>MSISSLLEKNIYNVHNKSNTLTNVPANPTGNTNTVWSNSNFTPPHLMYGASDITQAIGNISLTTGSFSLSLSGPWASPLVQNVAYTKINNLVNLTFPPFQANATSSAVINSAIGA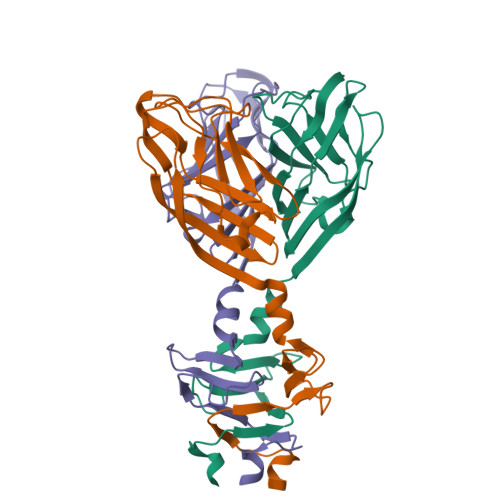LPADLRPTTNIQVDFEIFVIDDGNRPVNPGLITLLSNGQIVVYKDNNLGQFTTGIGGSGFNPFSITYMV[6x]>[6x]MSASDGQGMRAVILVGGFGTRLRPLTLTTPKPLVPFCNKPMIIHQIEA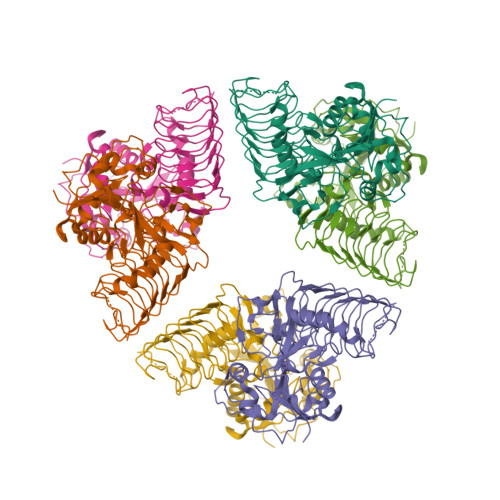LKAVGVTEVILAVAYRPEAMKEQMDEWSRKLGVSFVFSVEEEPLGTAGPLALARDILMQDDKPFFVLNSDVTCTFPMQELLDFHKAHGGEGTIMVSQVTQWEKYGVVVYSPQNYQIERFVEKPSRFLGDRINAGIYIFNKSILDRIPPRRASIEKEIFPAMAAEGQLYAFNLEGFWMDVGQPKDYILGMTKFIPSLVHGNRETEQLHTEAVEHQRGGRFTVIGASLIDPSAKIGDGAVIGPYASIGANCVIGESCRIDNAAILENSKVGKGTMVSRSIVGWNNRIGSWCHIKDISVLGDDVEVKDGVILIGTKVLPNKDVGEHRFEPGIIM>GPLGSVEEIRLPRAGGPLGLSIVGGSDHSSHPFGVQEPGVFISKVLPRGLAARSGLRVGDRILAVNGQD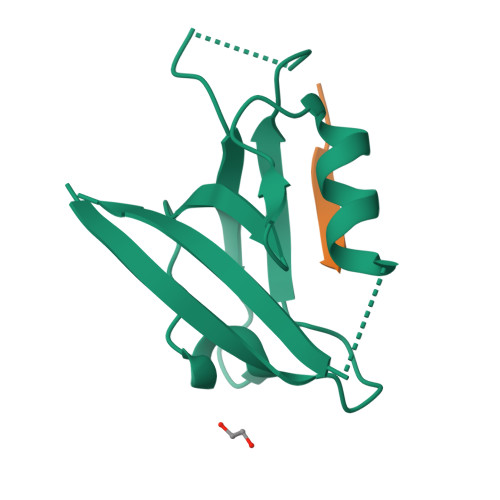VRDATHQEAVSALLRPCLELSLLVRRD[2x];>RLQSETSV[2x]> MRVTELIIDGFKSYAVRTVITGWDESFNAVTGLNGSGKSNILDAICFVLGITNMSTVRAQNLQDLIYKRGQAGVTKASVTIVFDNRDKKRSPIGFEEYATISVTRQIVLGGTTKYLINGHRAQQQTVQNLFQSVQLNINNPNFLIMQGRITKVLNMKPAEILAMIEEAAGTRMFEDRKEKALKTMAKKDLKLQEITELLADEIEPKLEKLRQEKRAFLDFQQTQSGGSGGSLRKKINPKVMNMIDSVEKKEMSLKHMMKTVLKDKHKIEETIATLDEYKRKALQETWEKVNGDFGQIFNELLPGSFAKLEPPEGKDLTDGLEVKVRL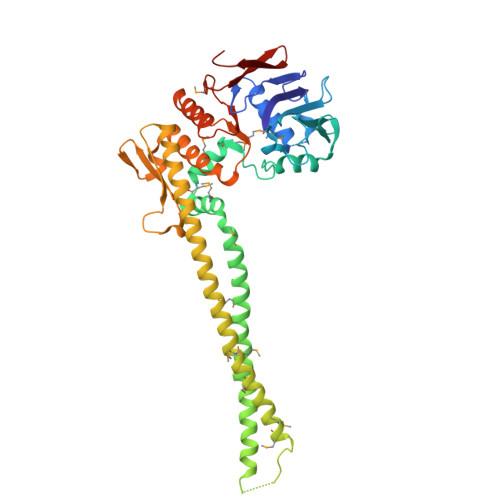GKVWKQSLTELSGGQRSLIALSLIMALLQFKPAPMYILDEVDAALDLSHTQNIGRLIKTRFKGSQFIVVSLKDGMFQNANRIFRVRFSEGTSVVQALTPADLK The CCR4–NOT complex plays a central role in the posttranscriptional regulation of gene expression by catalyzing the removal of the mRNA poly(A) tail, thereby repressing translation and promoting mRNA degradation. The CCR4–NOT complex is a multisubunit complex that assembles on the NOT1 scaffold protein, which consists of several α-helical domains that serve to dock the other subunits of the complex. NOT4 is an evolutionarily conserved E3 ubiquitin ligase that contains a RING domain, a linker region with coiled-coil propensity (CC), an RNA recognition motif (RRM) domain, and a C3H1-type zinc finger domain (ZNF). Assisted by alignments of metazoan NOT4 proteins, we uncovered a 23-amino-acid peptide motif in NOT4-C that binds to the CAF40 subunit of the CCR4–NOT complex and hence was termed the NOT4 CAF40-binding motif (CBM).

We obtained crystals—but only of a heterologous complex consisting of Hs CAF40 and the CBM of Dm NOT4. We obtained two distinct crystal forms, each with two crystallographically independent complexes per asymmetric unit and diffracting X-rays to a maximum resolution of 2.1 Å. CBM binding is highly similar among the four CAF40–CBM complexes, and therefore only one of them (polypeptide chains A and B from space group P212121) is described. Despite its highly negative overall charge (pI = 3.6), the Dm CBM interacts with Hs CAF40 primarily via hydrophobic contacts. It engages the concave surface of Hs CAF40, contacting residues from three parallel α helices (α5, α8, and α11) and burying a surface on Hs CAF40 of 842 Å2. Importantly, the very same surface of CAF40 was described previously to be engaged also by the CBMs of Roquin and Bam (Sgromo et al. 2017, 2018). Strikingly, however, whereas the CBMs of Roquin and Bam run in parallel to the α helices α5, α8, and α11, the CBM of NOT4 runs in an antiparallel fashion and hence is structurally and evolutionarily unrelated to the other two CBMs. At the C-terminal end of the CBM, the invariant Dm NOT4 E835 pins down the C-terminal half of the NOT4 α helix, using two hydrogen bonds to coordinate the free main chain nitrogens of Hs CAF40 A84 and H85 at the beginning of α helix α5 and compensating for the positive charge of the helix dipole. Additional specificity arises from an H bond between the side chains of Dm NOT4 T824 and Hs CAF40 T138 on α helix α8, which is deeply buried in the interface.

>[2x]GPHMLEREKIYQWINELSSPETRENALLELSKKRESVPDLAPMLWHSFGTIAALLQEIVNIYPSINPPTLTAHQSNRVCNALALLQCVASHPETRSAFLAAHIPLFLYPFLHTVSKTRPFEYLRLTSLGVIGALVKTDEQEVINFLLTTEIIPLCLRIMESGSELSKTVATFILQKILLDDTGLAYICQTYERFSHVAMILGKMVLQLSKEPSARLLKHVVRCYLRLSDNPRAREALRQCLPDQLKDTTFAQVLKDDTTTKRWLAQLVKNLQE;>DDDLGFDPFVETQKGLAELMENEVVQ[2x]> MEAVLNELVSVEDLLKFEKKFQSEKAAGSVSKSTQFEYAWCLVRSKYNDDIRKGIVLLEELLPKGSKEEQRDYVFYLAVGNYRLKEYE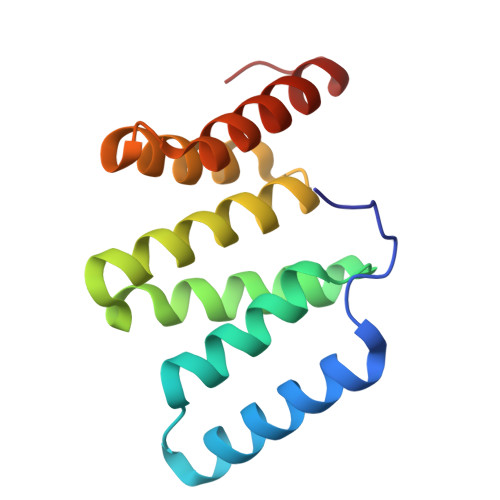KALKYVRGLLQTEPQNNQAKELERLIDKAMKKDGLVG>[4x]GPHMGSNRQELKDVCAPLEKDDIRRLSQAFHRFGIVTVTELIEPHTRKLVRAEADRLLDQYAERRDLRLATTDYTRRSMSVVPSETIAANSELVTGLYAHRELLAPLEAIAGERLHPCPKADEEFLITRQEQRGDTHG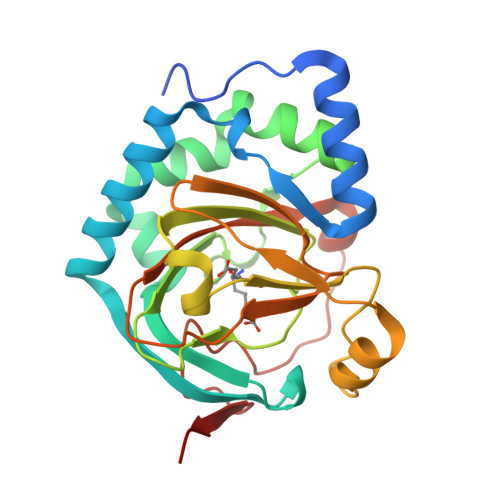WHWGDFSFALIWVLQAPPIDVGGLLQCVPHTTWDKASPQINRYLVENPIDTYHFESGDVYFLRTDTTLHRTIPLREDTTRIILNMTWAGERDLSRKLAADDRWWDNAEVSAARAIKD>MALLAEHLLKPLPADKQIETGPFLEAVSHLPPFFDCLGSPVFTPIKADISGNITKIKAVYDTNPAKFRTLQNILEVEKEMYGAEWPKVGATLALMWLKRGLRFIQVFLQSICDGERDENHPNLIRVNATKAYEMALKKYHGWIVQKIFQAALYAAPYKSDFLKALSKGQNVTEEECLEKIRLFLVNYTATIDVIYEMYTQMNAELNYKV[2x]

Mammalian glycolipid transfer proteins (GLTPs) are potential regulators of cell processes mediated by GSLs and display a unique architecture among lipid binding/transfer proteins. The 23–24-kDa GLTPs display absolute specificity for glycolipids, are highly conserved among mammals, and include plant and fungal orthologs that have been implicated in programmed cell death responses. The liganding site consists of a sugar headgroup recognition center that anchors the ceramide-linked sugar to the protein surface and a hydrophobic tunnel that accommodates the hydrocarbon chains of ceramide. Here we report crystal structures of human GLTP bound to GSLs of diverse acyl chain length, unsaturation, and sugar composition.

To search for additional conformational states related to the GLTP working cycle, we cocrystallized GLTP with a model compound, n-hexyl-β-d-glucoside, in which the sugar headgroup was β-linked to a single short (six-carbon) hydrocarbon chain, rather than a two-lipid chain ceramide moiety. GLTP binds the entire ligand at the protein surface, with the hydrophobic tunnel remaining closed and containing extraneous hydrocarbon for apo-GLTP. The sugar headgroup of n-hexyl-β-d-glucoside binds the GLTP recognition center in a manner similar to all GSL-GLTP complexes reported previously and in this paper. The same network of multiple specific interactions are observed between the n-hexyl-β-d-glucoside headgroup and the GLTP recognition center, with the only differences being the following: (1) the absence of hydrogen bonding between K55 and the glucosyl OH4 group because of its equatorial positioning and (2) the loss of hydrogen bonds involving ligands carrying the ceramide amide group and residues H140 and D48, which are now water bridged to each other. In apo-GLTP and the n-hexyl-β-d-glucoside–GLTP complex, the tunnel has collapsed, although the bottom (represented by cylinder 2) remains occupied by an extraneous hydrocarbon. A disruption of the H7/H29 stacking is observed in all apo-GLTP structures in which the H7 residue is resolved, including in our D48V apo-GLTP, as well as in our n-hexosyl glucoside–GLTP complex. In contrast, on n-hexyl-β-d-glucoside acquisition, there is only limited outwards movement of the α helix 2 N-terminal segment and adjacent loop L12, but no movement of the α helix 2 along its axis nor outward movement of α helix 6, keeping phenylalanine F148 in a swung-in position and allowing for only partial opening of the hydrophobic channel, in a fashion similar to that observed recently in GM3-His6-tagged bovine GLTP complex. Comparison of the apo-GLTP and the n-hexyl-β-d-glucoside–GLTP complex provides clear evidence that the recognition and anchoring of the sugar head triggers conformational rearrangements of the gate region, L12 loop.6-[(2~{R})-2-[(2-methylphenoxy)methyl]pyrrolidin-1-yl]-7~{H}-purine 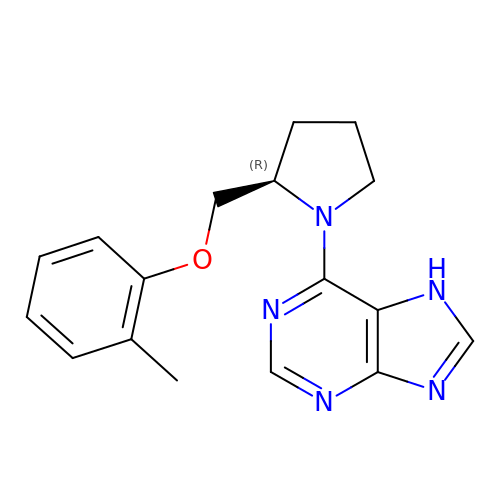| C17 H19 N5 O | SXTKECRQJMUZOI-CYBMUJFWSA-N(4R,6R,7S)-4,6,7-TRIHYDROXY-2-[(1E)-PROP-1-EN-1-YL]-4,5,6,7-TETRAHYDRO-1-BENZOTHIOPHENE-4-CARBOXYLIC 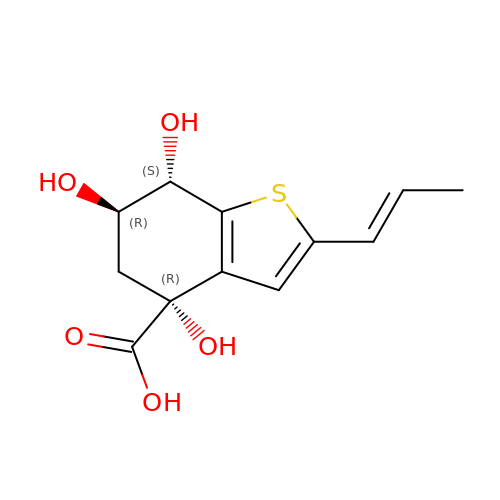ACID | C12 H14 O5 S | XBFFFFBWIVSOII-PJMUFDJCSA-N3-[5-(2-fluorophenyl)-1,2,4-oxadiazol-3-yl]benzoic acid | C15 H9 F N2 O3 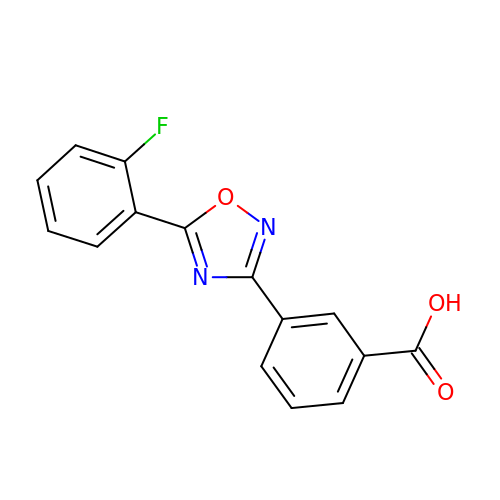| OOUGLTULBSNHNF-UHFFFAOYSA-N> FLTAVSSIDTFLPVLNEAKLQWPTSALAASSEELLGGYVGSQFYLQDGKYMQFQIAGSSNRCELRQMIPDGGSEIGWAVDDGTTHTATSSIVVPEQVDGVEEVTIMQIHSGEAPQLRISWIRSKSLDGVAYEDFIMSTVRIGTGDSSDNFVKTHLADRTAGAMSFQIDVKDSKLTITVNGNVVVNGQDLSFWDGTDSCYFKAGAYNNNPTSESATARIKFAALAWV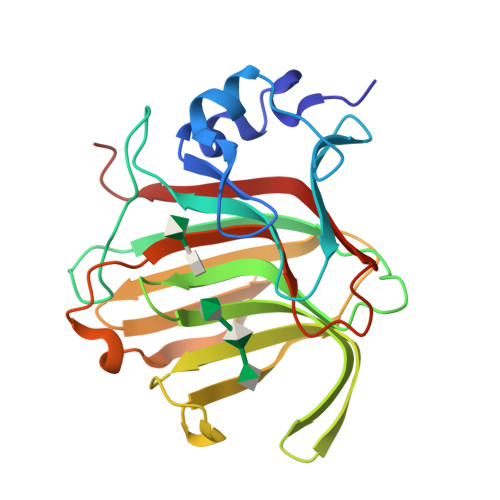DHHHH> STQNSSSVQDKQLQKVEEVPNNSEKALVKKLYDRYSKDTINGKSNKSRNWVYSERPLNENQVRIHLEGTYTVAGRVYTPKRNITL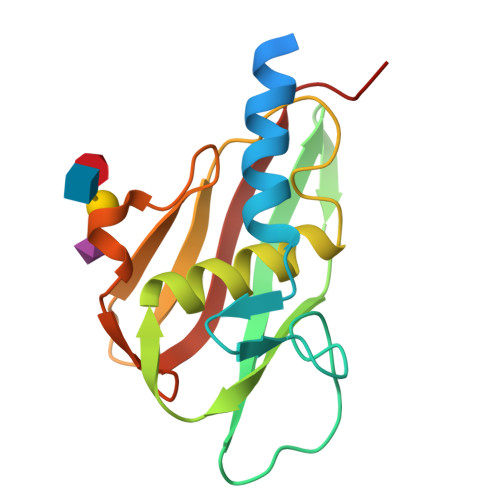NKEVVTLKELDHIIRFAHISYGLYMGEHLPKGNIVINTKNGGKYTLESHKELQKNRENVEINTDDIKNVTFELVKSVNDIEQV>[5x]MKITVVDLGNINVKYVGENKGRFSSKITNDYQSYEEGFQRVEYNGIKTYIGVGELSREFNKADRDYMAQLLYSLAKANTADTKEINLTLLLPIIQMKNKTRLIETLKGENFKFKFNGIDREIKINDLMVLPEGYASYYSLDIENKKGDVCILDLGSRTINICVLENAKIVKTNTIKLGSFDFYSKIKSLENAKGEDYIEEDIQRLIDNGLIKVDSKQYIEFLSDILNAVKPYVNLKTYNTIFTGGTSLMLKEYIEKLPLNKFKVHPNALTSNVDGAMEASKKVWN

ParMs generally exist on low-copy number plasmids where they contribute to plasmid segregation and stable inheritance. Here we report the discovery and characterization of two chromosome-encoded ParMs (cParMs) from the genomes of Desulfitobacterium hafniense (Dh-cParM1) and Clostridium botulinum (Cb-cParM). Both cParMs form filaments, exhibit nucleotide hydrolysis, and possess characteristic ParM subunit structures.

The 2D classification images of Cb-cParM polymerized with GTP appeared to show a mixture of two states. One state was similar to Cb-cParM polymerized with ATP, and the other was distinct. We tried polymerization with GTP for a shorter incubation time (1 min), which yielded the latter of the mixed states. The averaged images from the short incubation time, showed a more uniform diameter along each filament. Two maps were reconstructed from the second condition (GTP, 30 min), corresponding to the two groups in the 2D classification, class 1 and class 2, and one map from the short GTP incubation (1 min). The maps from class 2 with GTP (30 min) and the third condition (GTP, 1 min) were similar to each other, although the resolution was limited, suggesting that they were in the state before the phosphate release. The nucleotide-binding cleft was slightly more open in the models for class 2 with GTP and short incubation time with GTP, relative to the GDP state. The intra-strand interactions between subunits were very similar in the three models, except for a slight shift in the position of the adjacent subunit in the GDP state. The GTP (30 min) class 2 state and GTP (1 min) are equivalent in their inter-strand orientations and have fewer cross-strand contacts than observed in the GDP state, suggesting stabilization of the filament bound to GDP. Thus, there are two dramatically different Cb-cParM filament conformations: one comprised of loosely associated strands (likely to be bound to GTP or GDP-Pi); and the second formed by a closer association of the strands bound to GDP.> SNAMARKKNTSDQSRSQAANTPIAG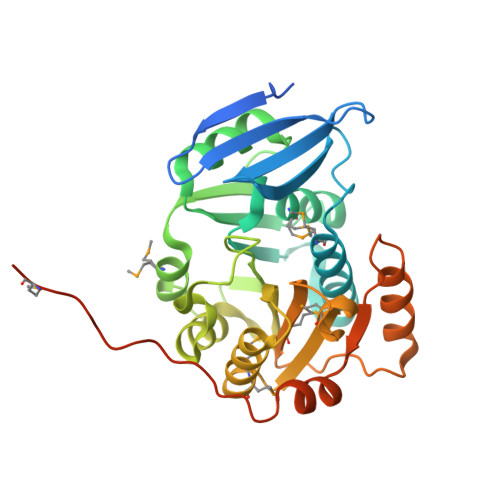TYEGEYSVIELEADSYTTDGWLISINGVPSSHIVLGQPQALEFEYMRWIATGARAFIDAHQDASKLRITHLGGGACTMARYFADVYPQSRNTVVELDAELARLSREWFDIPRAPRVKIRVDDARMVAESFTPASRDVIIRDVFAGAITPQNFTTVEFFEHCHRGLAPGGLYVANCGDHSDLRGAKSELAGMMEVFEHVAVIADPPMLKGRRYGNIILMGSDTEFFSSNSTEASAITRELLGGGVPAQYKDESWVRKFASGAQARHDGVSTLQMPSDTPQHPAETPEHSNTQP>[6x]MRGSHHHHHHMASMVDPRTPVIVGVGQFTERIDLDGYRGMSSVELATEAAKAALHDCGADADTVARAIDTVAGTRQFEISGPASAPLGVSSNYPRSVARNIGADPAHAVLEVIGGQSPQHLATEFGGKIAAGENDVVLIFGSENTSTLRHFSKAENKPDHSETVDGQLEDRGYGYDGIFDEYTIRHGLIGAPVQYGLLENARRAR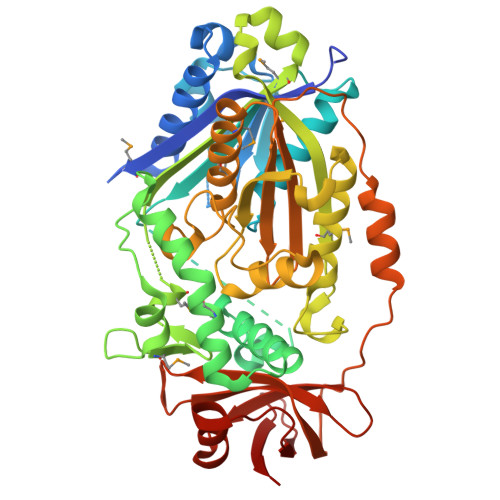LGLSVADYRLAMAELFAPFSKVAAKNPYSSAPTERSVEELLTVTASNRMIVDPYPRLMVARDQVNQGAALLMMSVESARKLGVPEEKWVYLRGHADMKEPKLLERADIGASPASVTAVNEALRVAGIGLDDVAAFDLYSCFPFPVFNICDGTGLATDDPRGLTLTGGLPFFGGLGNNYSMHGIAEAVNEMRDKPGQFALVGANGGIASKYSVGIYSTEPADWVADNSAQLQAEHDAQPKVAITEKADGTGTIETYTVRYDWTPHTGIIIGRLDDGSRFLAKTKDEDLVKLLSEGDPIGAKIVVTPGEKSNRAVLA> NEALARVEVAVLCLILLLALSGNACVLLALHTTRQKHSRLFFFMKHLSIADLVVAVFQVLPQLLWDITFRFYGPDLLCRLVKYLQLVGMFASTYLLLLMSLDRCLAICQPLRSLRRRTARLAVLATWLGCLVVSAPQVHIFSLREVADGVFDCWAVFIRPWGPKAYITWITLAVYIVPVIVLATCYGLIAFKIWQNLRLKTAAAAAAEAPEGAAAGDGGRVALARVSSVKLISKAKIRTVKMTFIIVLAFIVCWTPFFFVQMWSVWDANAPKEASAFIIVMLLASLNCCCKPWIYMLFMGHLFHGIDCSFWCCNESYLTGSRDERKKSLLSKFGMDEGVTFMFIGRFDRGQKGVDVLLKAIEILSSKKEFQEMRFIII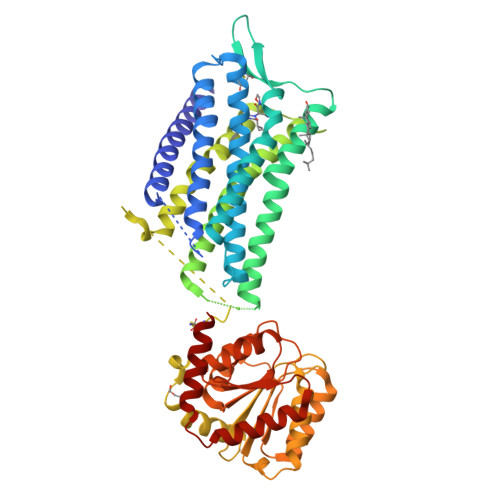GKGDPELEGWARSLEEKHGNVKVITEMLSREFVRELYGSVDFVIIPSYFEPFGLVALEAMCLGAIPIASAVGGLRDIITNETGILVKAGDPGELANAILKALELSRSDLSKFRENCKKRAMSFS>MLTNSEKSRFFLADLTGEVQSIPNTYGYISGLGLFRSAPQTQTTFLMDLTDWDISLLDAVDRTSRKAETSAPERVRQISFPMMYFKEVESITPDEIQGVRQPGTANELTTEAVVRAKKLMKIRTKFDITREFLFMQALKGKVIDANGVLYADLYKQFDVTKKTIYFDLDNPNSDIDAHIEDLRMHMEDEAKTGTVINGEEIHIVVDRTFFSKLIKHPKIRDAYLAQQTPLAWQQITGSLRTGGTDGVQAHMNRFYYGGVVFVQYNGKFKDKRGKTHTLVSIDGVSDTNVGVGHAFPNVAMLGEANNIFEVAYAPCPKMGYANTLGQELYVFEYEKDRDEGIDFEAHSYMLPYCTRPQLLVDVRSDAE[9x];>[9x]MAYQGFTKLGEREPLNDIILWEEITPTGHSRKEYAPVASTEYRVGEVLKADGSKVAAGQEAQADSVCIVNFYADLQLSYHGQLKVVGIYRDAELKDLLKLESGVDAAAVKSALKAKGIDFVPTGL;> MIKAKTYPDFKEFVKDFVANVKAGKRYDFRKYQEAVLPLTYSSPWPESDIPEVTDFNYTPDYTVPFSEELLYSVGAQMRTADFFMDLQYAIINGKDVDTVYCEWLARVKPFSMLNAKLKDSAQPPVITTQPTGGAVNEGSAINLSIVATNATSYQWKKGSSDISGATSATYTKAGAVPADAGSYTCVVTNDVGSTTSDAAVITINPLPVITTQPTSKAVNESSTLTLSVVATGATSYQWKKNGTNISGATSATYSKANAKTTDAGSYTC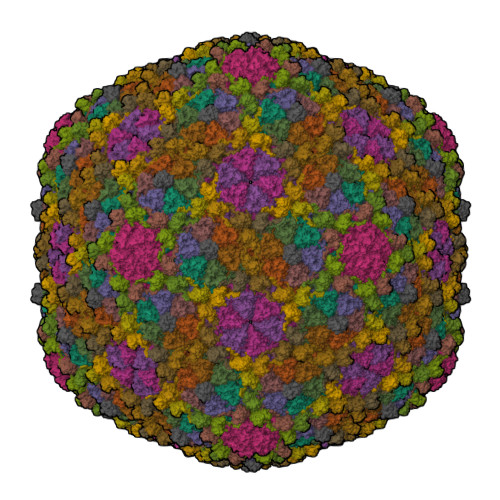VVTNAVGSVTSNAATVTINPLPVITVQPQDQDLTVGQTLTISITATGATGYQWRKGNSNISGATSATYTKASVTTADDGNYDCVVTNAVGSVTSHQAKVQVTA> MTETPATPTGLPTARAAGCPFDPPPGLAALRDRAPLTRMEFPNGHVGWLATGHAVVR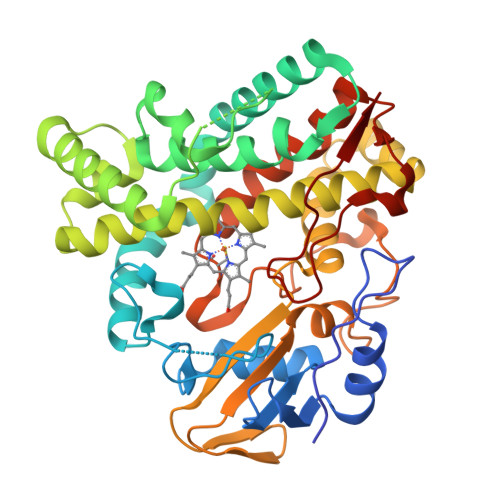AVLADPRFSHRNDRRHWPLADIGRGFPPLPGDMLHIDPPDHTRYRKLLAGKFTMRRMRRLTGSAQEIVAGKLDAMERHGGPLDLLEFFARPVPTLMVCALLGVPLQDRATFHPPVRGTDDAAAVEADVAAYVEMTYADMQEYFRKLVAAKRAAPADDLLSDLTTSDLTEDELVGLCAVMMHAGVDSTSNMLALGTWALLERPDQLAALRERPDLADRAVEELMRYMSVVHTGSRAALEDVELAGEVVRAGESVAFSVQAANRDPARFADPDTLDIRRGAVGHLGFGYGVHQCLGMQLARVEMRVAFPALFARFPALRLAVPAGDVPMRDDLVIPYGVHRLPVTW> PQNSQLTWKQGRQLLRQYLQEVGYT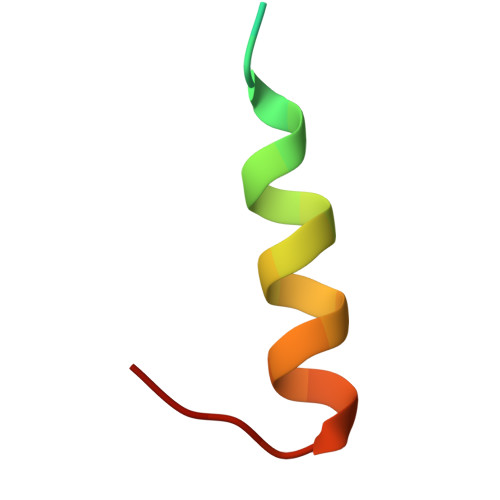D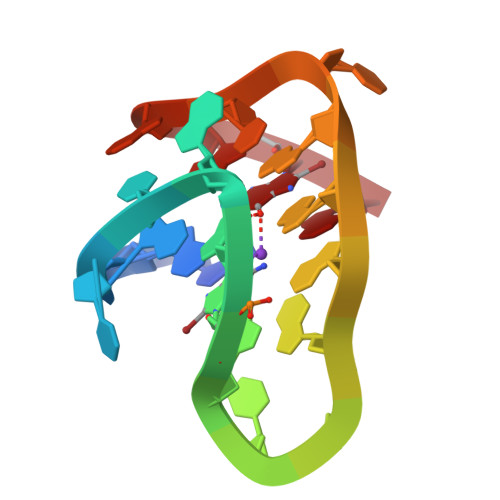> GGGTTAGGGTTAGGGTTAGGG>MSTLNKHISIPKDMSSKDDLDFHFLREEGIRYIKELGSNFWTDYNTHDPGITMLEVLCYAISDLGNRINIPIEDLIANEEGGVKGQFYKVQEILPSAPTSELDLRKLFIDIEGIKNCWIKRERVTVFADLKNQKLSYEKTIWEDLKENQKAQFDLKGLYRILVETEDADKVLSESLEKAVFTKFHANRNLCEDLIKVEKVATEPISVCANVEVAPEADEELIHAQILIAIEDYLAPSPRHYSLKQMVDKGYTMDEIFEGPFLENGFIDTVELKASELRKEVRLSDIINIIMSIDGVKIVKEITLGNCDENDGIENNQWVICIPENKKPKLCKKTTINYFKGILPINLNPVRVDNHKSKILASRLENDLKAKDDLEPAIPQGTFADWGEYSSIQHEFPETYGISDIGLPPKLGVKRAVLARQLKGYLLFFDQILASYFEHLSKIKSLLSLDQGPSFTYFTQAIKDIKDVEELFKDPTLLENDEELTKSLIGKLDDTIERRNQLMDHLIARFAENFSSYAFLMKFLYGESTDEIVLQDKQSFLREYKEISRERGEGFNFYEQSNDNLWDTLNVSGAQKRISKLVGVKDYSRRNLSDTAVEIYRYEHVDGNWVYRWRIRDENGKVLLSATTSYPTYNSAGNEMYFAILKILETPLSDLEKLLEVNFRNENEAGSFHFHKAATSNKFSFDIINPVIDSESSSDFIVAKQYTYYPDRTQAVLGAISLLNFIKYTFTEEGIYLVEHILLRPSPLDPEYLAMQTDAGKEYIEGNFLPFCSDDYENCKMIDPYSFRVSIVLPGFTYRFANKDFRDYLENLIREELPAHIVAKICWIGYRKGEEPELFQEDVENPETPIFKENQLEIFEKAYKNYLFELTDIHKRKGFIASMNKYNQVLNEMTSSLTGLHTIYPTGRLYDCEDEEEELDGKLILGKTNLGTL[6x];>[6x]MSENCNHIVTTLKRDGTGRRDLLDPKLAPESVQLQDFELSDWLIFALNFARKIHFFPSDLANEPLGDWRNFFSTIVSDKTLISDIENLDDFEKLRGNIEEFLAAYDQSGKLTPHLTLFVSFLKLLETSKKRFNQLTKRHLDFYYQEILHLEKQALSPDHVFLIFELAKNVSQEKLDEGTEVDGGKDDTGKKNTYLTSFETVLNKTKVGQLKSLYNEISVEKEEIKELNTPISTGTFVMAPMANSFDGLGEDFPKGSEKWWPFGYTKICNASTVLPALPKARLGCSISSKLLKLSEGTRDIILEFTFNKPILPNGEDYTALNKAMSIELTGEKGWIAGLPMTLKSDSGINSGSKKMKLSLTLDSEQPAVVPYQTELHEGSYEVDEPLLRVLFKTNEKEGYNLYRLFNENVLTDLKITVEVSDITSVQLENDLGVLNPQKPFFPFGPRPIKGSSFIVKYPEAMEKPVTAISYQMDYLNLPENLVNHYSAYTIGDDEPLVSDMDYFSVKSFPKSSNDSDQLFSEKSGGGYESDFEFQIENGVWESGLKKELKISLERSFLHEKYAHYFTLVAISKDTDPTIELLPNEPYAPLAENLVLGYTAISSIDFSSSSSENQVSLIHEMPFGFQQVFTPGDTDNSLYLVPDYCHGGELYIGLENGKNLQQVTLLLQFLEGSENPDITDIFTGNQKIKWQYLSQNQWQDFQSGEIIQNQTPRFLKSGIFQFSIPKQANLDNTVLPPGYHWIKASMVKPFDVVSQLINIHAQAVEAVFEDQGSSGNHLEKGLPAETISKLQERLSWIKSIQQPYPSTKGKAQESDEDYYRRVSERLRHKKRAITLWDYEHLILQKFPKVYKVKCLNHTCSSSFQSPGNATLILVPDTVQQSVFDIYQPRVSQGTLNDVAAFVNELNSFHVQAKVINPNYEEVKVDVKVKFREGLDVSFYLTKVKEDIKKFLSPWAYDQESSVEFGVTLHRSQMIHYLEQLTYVDYITDLRLLKRQAGSSPCNPIFIETTEKEYIQPSNPKSILVSAKEHLVTPITQNCSSISLNNEEECQH;>MSEGKLEKLRIVAYKDSKFSDEVENGEFITLLNPEKYKFQYRVEQNEDQASGTSSAPIRFNKILPQTLEFDFLFDRTGVIAGYEVTEDGIINDIDHFKKVVYDYNGEKHKPNYLMITWGSLLFKGYLKEMDIEYKLFRPDGTPIRAMATTKIGEFVEEELRTAQENNQSPDMSHYRTVKEGDTLPLMTYRIYGDSKYYLEVAKANGLTNFRRLKTGTELIFPPLQKQK[6x];>MMEKSKDFLGTGWGFPPEFETSIGQVKTTSGVEDIQKSLEILFSTKIGERIMQPTYGCNLDELLFSPINRTLKTYVIELIKNAILYHEPRIDPEKIDITQGNEIEGELLIHLQYIVRATNSRKNMVYPFYLEEGTNI[6x];>MATYYPPSSFHFLVEFTGIDAKNNDHEFQSVSGLSVDIDTEEFAEGGENRFKHKFPVKTKYPNLVLKRGVLVDSKVISWCRDAIEDFEFKPIDLTVKLLNEEHQPLMTWNVVHAYPVKWSVEDFNAQESKMAIESVELSYNYFKTIV[6x];>[6x]MATYKTPGVYIEEITKFPPSVAQVETAIPAFIGYTQFARTKPSVDSDDLILKPKRISSLLDFTTYYGGAQNEQGITVKLTDTLIEGAENRTINVPEPTFKSPYLMFYSLQMYFANGGGPCYIVSTGVYDDWSDSETPPTINFSDLESGLAVIRKEDEPTLLLFPDATNLPTDDEFYSLYNSALMQCNDLQDRFTILDTYSDQTYNDGVEDLDPIPALRNGINLTKDYLKYGAAYYPFVQTILNYQYSADEIVIQHLSYNPNAIATALDNLNAVNGPTFIDAILDDLRDLSLPDISGEISDAVGFMYDDVDGFDIDGTFTTNSVKVANFASLVESVLSTLNELIDAKEEINKDVNSAIASSEEDNAIKTAISDALDVFNEDFEGADKIESVAKNLSDLLIKIKQADTNTKVENVLSINALNFSAEFEKLLTYDVNTGLTASVTLDLFANIGTRLDDIIAAVSAAEPIDVNNGKLNGRLLSDIEPLDNATYNTILLEINSHKVTLPPSSSMAGAYARVDNDRGVWKSPANIGLNYVSKPSVTVSHEEQESMNVHGTGKSVNAIRSFVGKGTLVWGARTLAGNDNEWRYISVRRFFNMAEESIKKATEQFVFEPNDGNTWVRVRAMIENFLILQWRAGALAGAKPEHAFYVKVGLGQTMTAQDILEGNMNVEIGLAVVRPAEFIILKFSHKMQES;>MSYPLSKFHFSVEWGGTKIGFTEVSGLDLETEIIEYRHGASPEYSKIKMPGMQKFSNITLKRGTFKSDNEYFQWYNTINLNKVERRDLTISLLNEEHEPVVTWKVKNAWPLKVQSTDLKGDGNEVAIESMELAHEGLVIQNE[6x];>MNNSGTIETSQSVDRVTHKIL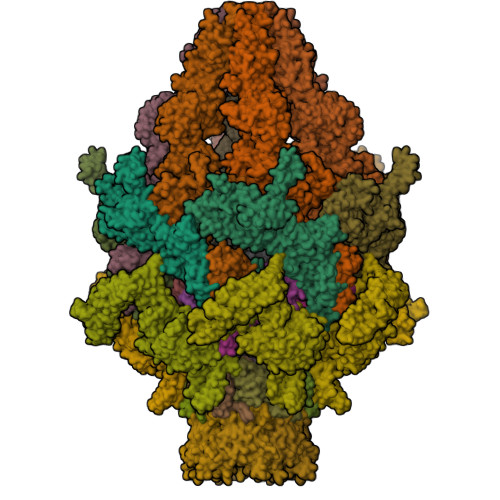IDGSEIPGTYQVKSIQVTKEVNRIPTARLVILDGDAAERDFKVSNSDHFVPGKEIEITVGYHSDDETIFKGVVIRQNLKIRNNQSILIVESRDMAVKMTLRRKSKYFYELSDSDILEELISNHGLEADVASTENQHTELVQYDVTDWDFMMLRLQANGLLCLVDDGKVSIQKPDLSSEALETVTFGATILEFDAEMDARNQLPKVVSQAWNMSDQELLEKEGVDPSLETNGNISSSDLASLFDQEEEVLRHGGSKKDGSLQEWANAKWTFQQLAKTRGRIKFQGIPTVKPGVNLLLEGVGDRFNGKVFITGVNHQISEGNWTVDAQFGLNPEWFSESESNIHTPPAAGLTAAISGLHVGLVTDLEDPDGEDRIKVKIPIINNEEEGVWCRQAFPDAGNERGITFRPEIEDEVIVGFINEDPNDAVVLGMLHSSANPNPIEASNDNHEKGIQTRSGIKMIFNDEKSILQIETPTGNLVTLDDDAGSITIEDQNGNKTVMDSDGITMESAKDMNLKASGDINLEGTNVNIKANAEFKAEGSAGAEVSTSAVAVLKGSLVQIN[3x];>MPIEIKELHIKITVDDSNNAGRGGASSGEDKQQLVAQCVEQVLDVLKSQKER[3x]>[4x]MFRNHASRITAAAAPWVLRTACRQKSDAKTPVWGHTQLNRLSFLETVPVVPLRVSDESSEDRPTWSLPDIENVAITHKKPNGLVDTLAYRSVRTCRWLFDTFSLYRFGSITESKVISRCLFLETVAGVPGMVGGMLRHLSSLRYMTRDKGWINTLLVEAENERMHLMTFIELRQPGLPLRVSIIITQAIMYLFLLVAYVISPRFVHRFVGYLEEEAVITYTGVMRAIDEGRLRPTKNDVPEV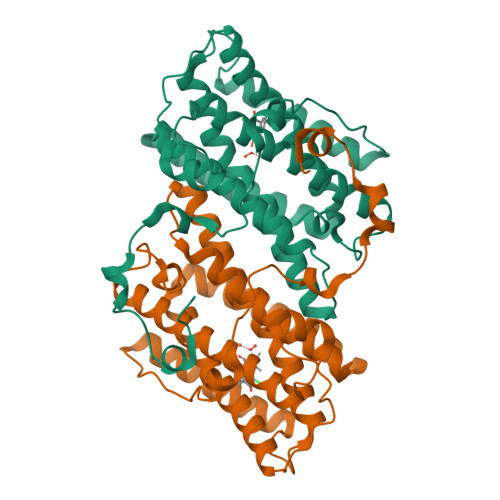ARVYWNLSKNATFRDLINVIRADEAEHRVVNHTFADMHEKRLQNSVNPFVVLKKNPEEMYSNQPSGKTRTDFGSEGAKTASNVNKHV TDIF consists of 12 amino acids including two hydroxyproline residues, and is encoded by the CLE41 and CLE44 genes in Arabidopsis9. TDIF is secreted from the phloem and is perceived by its specific receptor, TDR/PXY (TDIF receptor/phloem intercalated with xylem), which is located on the procambial cell membrane. TDR belongs to the LRR-RK class XI subfamily, and consists of the extracellular LRR domain and the cytoplasmic kinase domain10. TDR recognizes TDIF by its extracellular LRR domain, and activates the intracellular GSK3 pathway to suppress the transcription factor BES1, which promotes cellular differentiation into tracheary elements.

To improve the solution behaviour of the TDR extracellular domain, we introduced mutations to two less-conserved cysteine residues (C259A/C540S), and performed the crystallization screening using the lysine methylated C259A/C540S TDR mutant20. Finally, we obtained the crystals of the TDR–TDIF complex, which diffracted X-rays up to 3.0 Å resolution. The extracellular domain of TDR forms a twisted right-handed superhelix composed of 22 LRRs and N-terminal (residues 34–81) and C-terminal (residues 609–637) capping domains. In the crystal structure, we observed the electron densities for the 11 glycan chains attached to the Asn side chains in the LRR domains, although their biological functions are unknown. The electron density of TDIF is clearly defined on the concave surface of LRR4–LRR15 of TDR. TDIF adopts an extended conformation, with a kink around Gly6–Hyp7 at the middle of the peptide. In the middle part, the kink around Gly6–Hyp7 is recognized by the pocket formed by Asp255 (LRR8), Phe279 (LRR9), Phe281 (LRR9) and Trp325 (LRR11) of TDR, in a shape-complementary manner. In the N-terminal part, the imidazole nitrogen of His1 of TDIF hydrogen bonds with the main-chain carbonyl groups of Ser187 (LRR5) and Gly210 (LRR6), and the N-terminal amino group and the carbonyl group of His1 of TDIF form further hydrogen bonds with the hydroxyl group of Ser162 (LRR4) of TDR. At the C-terminal part, the Asn12 side-chain carbonyl group of TDIF hydrogen bonds with the side chains of Arg421 and Arg423 of TDR. Collectively, the present crystal structure suggests that the central kink of the CLE peptides, including TDIF, offers a common platform for the recognition by the CLE peptide receptors, while the N- and C-terminal parts provide the sequence-specific readout for the cognate CLE receptors.

> KFSPQLLSLLSLKTSLSGPPSAFQDWKVPVNGQNDAVWCSWSGVVCDNVTAQVISLDLSHRNLSGRIPIQIRYLSSLLYLNLSGNSLEGSFPTSIFDLTKLTTLDISRNSFDSSFPPGISKLKFLKVFNAFSNNFEGLLPSDVSRLRFLEELNFGGSYFEGEIPAAYGGLQRLKFIHLAGNVLGGKLPPRLGLLTELQHMEIGYNHFNGNIPSEFALLSNLKYFDVSNASLSGSLPQELGNLSNLETLFLFQNGFTGEIPESYSNLKSLKLLDFSSNQLSGSIPSGFSTLKNLTWLSLISNNLSGEVPEGIGELPELTTLFLWNNNFTGVLPHKLGSNGKLETMDVSNNSFTGTIPSSLCHGNKLYKLILFSNMFEGELPKSLTRCESLWRFRSQNNRLNGTIPIGFGSLRNLTFVDLSNNRFTDQIPADFATAPVLQYLNLSTNFFHRKLPENIWKAPNLQIFSASFSNLIGEIPNYVGCKSFYRIELQGNSLNGTIPWDIGHCEKLLSLNLSQNHLNGIIPWEISTLPSIADVDLSHNLLTGTIPSDFGSSKTITTFNVSYNQLIGPIPSGSFAHLNPSFFSSNEGLCGDLVGKPCNSDSGLEVL;> HEVPSGPNPISN>[2x]SFKDLN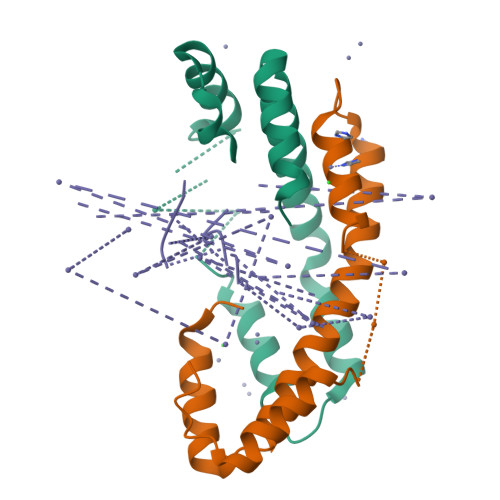LTDAQKQQIREIMKGQRDQMKRPPLEERRAMHDIIASDTFDKVKAEAQIAKMEEQRKANMLAHMETQNKIYNILTPEQKKQFNANFEKRLT;> SISDYTEAEFVQLLKEIEKENVAATDDVLDVLLEHFVKIT> 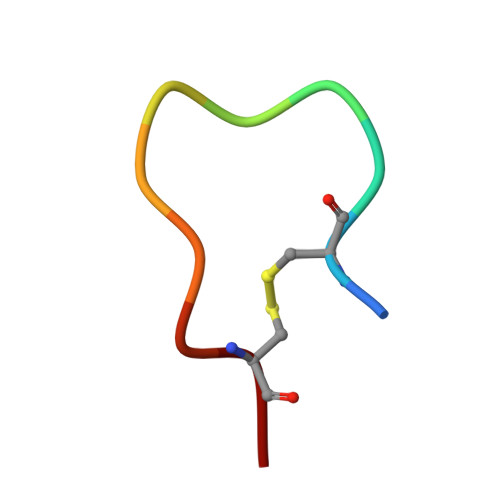KCPGRVVGGCK[[(2~{R},3~{S},4~{R},5~{R})-5-[4-[(1~{S},3~{a}~{S},3~{b}~{S},5~{a}~{R},8~{S},9~{a}~{R},9~{b}~{S},11~{a}~{S})-1-(~{tert}-butylcarbamoyl)-9~{a},11~{a}-dimethyl-7-oxidanylidene-1,2,3,3~{a},3~{b},4,5,5~{a},6,8,9,9~{b},10,11-tetradecahydroindeno[5,4-f]quinolin-8-yl]-3-aminocarbonyl-4~{H}-pyridin-1-yl]-3,4-bis(oxidanyl)oxolan-2-yl]methoxy-oxidanyl-phosphoryl] [(2~{R},3~{R},4~{R},5~{R})-5-(6-aminopurin-9-yl)-3-oxidanyl-4-phosphonooxy-oxolan-2-yl]methyl 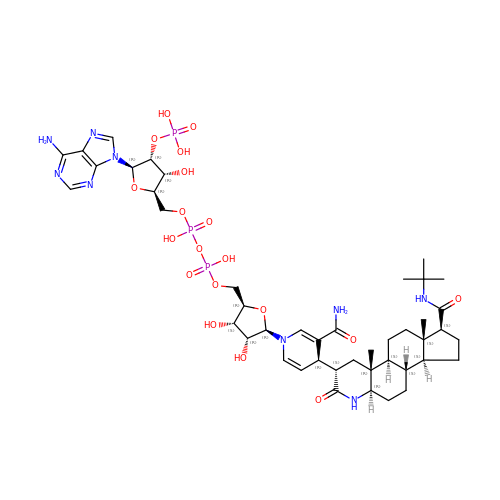hydrogen phosphate | C44 H66 N9 O19 P3 | SBPCUEDRMWGINQ-DAPYLVMHSA-N>MPSVYGARLTTFEDEEKESEYGYVRKVSGPVVIADGMNGAAMYELVRVGHDNLIGEIIRLEGDSATIQVYEETAGLMVNDPVLRTHKPLSVELGPGILGNIFDGIQRPLKTIAIRSGDVYIPRGVSVPALDKDTLWEFQPKKIGEGDLLTGGDLYATVFENSLMQHHVALPPDAMGKVTYVAPAGQYSLKDTVLELEFQGVKKSFTMLQAWPVRTPRPVSSKLAADTPLLTGQRVLDALFPSVLGGTCAIPGAFGCGKTVISQALSKYSNSDTVVYVGCGERGNEMAEVLMDFPQLTMTLPDGREESVMKRTTLVANTSNMPVAAREASIYTGITIAEYFRDMGYNVSMMADSTSRWAEALREISGRLAEMPADSGYPAYLAARLASFYERAGKVKCLGGPERTGSVTIVGAVSPPGGDFSDPVTSATLSIVQVFWGLDKKLAQRKHFPSVNWLISYSKYSTALESFYEQFDPDFINIRTKAREVLQREDDLNEIVQLVGKDALAEGDKITLETAKLLREDYLAQNAFTPYDKFCPFYKSVWMMRNIIHFYNLANQAVEKGAGMDGQKITYTLIKHRLGDLFYRLVSQKFEDPAEGEPALVAKFKKLHEDLTAGFRALEDETR[3x];>MGVAQNNVDMEEGTLEVAMEYRTVTGVAGPLVILDKVKGPKYYEIVNIRLGDGTMRRGQVLEVDGEKAVVQVFEGTSGIDNKFTTVQFTGEVLKTPVSLDMLGRIFNGSGKPIDNGPPILPEAYLDISGSSINPSERTYPEEMIQTGISTIDVMNSIARGQKIPLFSAAGLPHNEIAAQICRQAGLVKRLEKTDNLLEDGEEDNFAIVFAAMGVNMETAQFFKRDFEENGSMERVTLFLNLANDPTIERIITPRIALTTAEYLAYECGKHVLVILTDMSSYADALREVSAAREEVPGRRGYPGYMYTDLAQIYERAGRIEGRKGSITQIPILTMPNDDITHPTPDLTGYITEGQIYIDRQLQNRQIYPPINVLPSLSRLMKSAIGEGMTRRDHSDVSNQLYANYAIGKDVQAMKAVVGEEALSSEDLLYLEFLDKFERKFVAQGAYDSRNIFQSLDLAWTLLRIFPRELLHRIPGKTLDQYYSRDAAN[3x];>MNDADVSKQIQQMVRFIRQEAEEKANEISVSAEEEFNIEKLQLVEAEKKKIRQEYERKEKQVEIRKKIEYSMQLNASRIKVLQAQDDLVSNMMEAASKEVLNVSRDHNSYKKLLKGLIVQSLLRLKEPAVLLRCRKDDHHLVESVLESAKEEYAQKLQVHPPEIIVDHHIYLPPGPGHHNAHGPSCSGGVVVASRDGKIVCENTLDARLDVVFRKKLPEIRKQLVSQVAA[3x];>[3x]MASNRGHGGIQQLLAAEQEAQHIVAAARNAKMARLRQAKEEAEREIAEHRAQVEREFQRKLAESSGDSGANVKRLEQETEVKIHHLNAGAEKIQYDVVQMLLKHVTTVKN;> MAQNQRLTVVPTVTMLGVMKSRLVGATRGHALLKKKSDALTVQFRQILKNIVTTKESMGEVMKDSSFALIEAKYVAGENIKHIVLENVQNASIKVRSRQENIAGVKIPKFEYFTDGETKNDLTGLARGGQQVQQCRAAYVKAIELLVELASLQTSFLTLDEAIKTTNRRVNALENVVKPRLENTITYIKGELDELEREDFFRLKKIQGYKKREIERQLASSKQFVEEQFAEKVSLQKGISIKSAQNLLSAGEKDEDIIF;> MAGRAQIPTKSSALIAMIADEDTVTGFLLAGVGNVDLRRKTNYLIVDSKTTVKAIEDAFKEFTTKEDIAIVLISQYVANMIRFLVDSYNKPIPAILEIPSKDHPYDPAHDSVLSRVKNLFSAESVASGRR;> MASRYWVVSLPVQNSAASVWNRLQEQISKHSFDTPLYRFNIPNLRVGTLDSLLALSDDLVKSNSFVESVSHKIRRQIEELERVSGIESSSLSVDGVPVDTYLTRFVWDEAKYPTMSPLREIVDGIHTLVAKIEDDLKVRVAEYNNVRSQLNAINRKQSGSLAVRDLSNLVKPEDIITSEHLVTLLAVVPKYSQKDWLASYETLTSYVVPRSSKLLYEDNEYALYTVTLFGRVADNFRIAAREKGFQIRDFEYSSEAQESRNQELEKLVHDQESLRSSLLQWCYTSYGEVFSSWMHFCAVRVFAESILRYGLPPSFLACVLAPSVKGEKKVRSILEELCGNANSTFWKSEDDGGMMAGLGGDADSHPYVSFTINLV;> MDHAELTTEQVLKRDI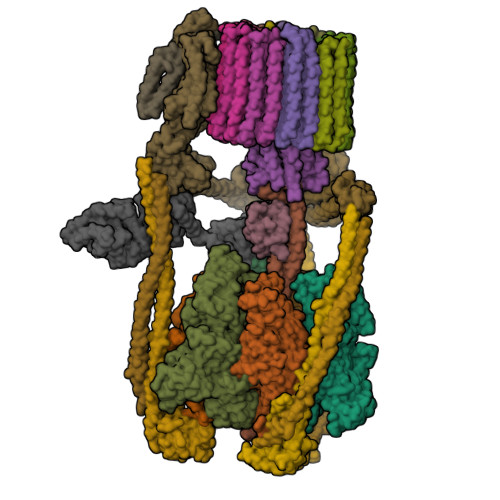PWETYMTTKLISGTGLQLLRRYDNRSESHRAQLLDDDGPSYVRVFVSILRDIYKEETVEYVLALIDEMLTANPKRARLFHDKSLASEDTYEPFLRLLWKGNWFIQEKSCKILASIVSARPKPQDRFFANGEASNSKSKSTTIDDVLKLLVEWLCAQLKKPSHPSRGVPVAINCLAALLKEPMVRSSFVQADGVKLLTPLISPASTQQSIQLLYETCLCVWLLSYYEPAVEYLATTRTLPRLIDVVKSSTKEKVVRVVVLILRNLLPKGNFAAQMIDLGLPQVVQSLKAQAWSDEDLLEGLNQLEEGLKDNIKRLSSFDKYKQEVLLGHLDWSPMHKDPLFWRDNITNFEENDFQILRVLLTILDTSSDPRALAVACFDLSQFIQYHPAGRVIVTDLKAKERVMKLMNHENTEVTKSALLCIQRLFLGAKYASFLQA;> MAELQSGGGGGCCPPMDLFRSEPMQLVQIIIPIESAHLTVSYLGELGLLQFKDLNSEKSPFQRTYAAQIKKCAEMARKLRFFKEQMLKAGILSSVKSTTRADNNTDDLEVKLGDLEAELVEINANGDKLQRAHSELVEYKLVLQKAGEFFSSALTSAAAQQREMESQQTGEMTIETPLLTDKEMSADPSKQIKLGFIAGLVPREKSMSFERMLFRATRGNVFLRQAVVDEPVVDPVSGEKMEKNVFVVFYSGERAKNKILKICDAFGANRYPFNEEFDKQAQAISEVSGRLSELKTTLDAGLLHRGNLLQTIGDQFEQWNLLVKREKSIYHTLNMLSLDVTKKCLVGEGWSPVFATKQIQDALERAAFDSNSQVGAIFQVLHTKESPPTYFRTNKFTSAFQEIVDAYGVAKYREANPGVFTIVTFPFLFAVMFGDWGHGICLLLGTLVLIVREKKLASQKLDDITDMTFGGRYVILMMALFSIYTGLIYNEFFSVPFEIFSHSAYACRDLSCSEATTVGLIKVRDTYPFGVDPVWHGSRSELPFLNSLKMKMSILLGVAQMNLGIILSYFNATFFRIGVNIWCQFIPQIIFLNSLFGYLSLLIILKWITGSQADLYHVMIYMFLSPTDELGDNQLFPGQKTAQLVLLLLAFVSVPWMLLPKPFILKMQHQDRHQGQSYEALQSTDESLQPDTNHDSHGHEEFEFSEVFVHQMIHTIEFVLGAVSNTASYLRLWALSLAHSELSSVFYEKVLLLAWGYNNILILIVGIIVFIFATVGVLLVMETLSAFLHALRLHWVEFQNKFYEGDGYKFSPFSFALLDDEDE;> MSGSVMLGESSSWSRALVKISPYTFSAIGIAVAIGVSVLGAAWGIYITGSSLIGAAIKAPRITSKNLISVIFCEAVAIYGVIVAIILQTKLESVPASQIYAPESLRAGYAIFASGIIVGFANLVCGLCVGIIGSSCALSDAQNSSLFVKILVIEIFGSALGLFGVIVGIIMSAQASWPAKPV;> MYGFEAMTFNIHGGYLEAIVRGYRAGLLTAADYNNLCQCETLDDIKMHLSATEYGPYLQNEPSPLHTTTIVEKCTLKLVDEYKHMLCQATEPLSTFLEYITYGHMIDNVVLIVTGTLHERDVQELLEKCHPLGMFDSIATLAVAQNMRELYRLVLVDTPLAPYFSECITSEDLDDMNIEIMRNTLYKAYLEDFYKFCQKLGGATAEIMSDLLAFEADRRAVNITINSIGTELTRDDRRKLYSNFGLLYPYGHEELAVCEDIDQVRGVMEKYPPYQSIFSKLSYGESQMLDKAFYEEEVKRLCLAFEQQFHYGVFFAYMRLREQEIRNLMWISECVAQNQKSRVHDSVVFIF;> MGFLVTTLVFLVIGIIASLCTRICCNRGPSTNLLHLTLVITATVSCWMMWAIVYLAQMKPLIVPILSEEE;>MSTFSGDETAPFFGFLGAAAALVFSCMGAAYGTAKSGVGVASMGVMRPELVMKSIVPVVMAGVLGIYGLIIAVIISTGINPKAKSYYLFDGYAHLSSGLACGLAGLSAGMAIGIVGDAGVRANAQQPKLFVGMILILIFAEALALYGLIVGIILSSRAGQSRAE[9x]Intraflagellar transport (IFT) trains, the polymers composed of two multi-subunit complexes, IFT-A and IFT-B, carry out bidirectional intracellular transport in cilia, vital for cilia biogenesis and signaling. The IFT-A complex is composed of six subunits (IFT144, IFT140, IFT122, IFT121, IFT139 and IFT43), mediating both the retrograde trafficking (toward the base) driven by the dynein-1b and the ciliary import of various membrane proteins across the ciliary gate. Here, we purified the IFT-A complex from protozoa Tetrahymena thermophila and determined the cryo-EM structures of the IFT-A complex and its subassemblies at a resolution range of 3.6 to 8.8 Å. Analysis of these structures reveal that the apo IFT-A complex is composed of two rigid structural modules, the head and base modules, and presents two distinct–elongated and folded states in solutions, the latter of which was not identified in recent IFT-A structural studies.

In particular, IFT144, IFT140, IFT122 and IFT121, share the same domain organization, from the N- to the C-termini encompassing two tandem WD40 β-propellers (WDs), an array of 12 to 20 TPRs and, except for IFT140, a zinc binding domain (ZBD). These four subunits are distributed into the two modules; the head module consists of IFT140, IFT144 and the C-terminal half of IFT122 (IFT122C, 706-1246), whereas the base module consists of IFT121, the N-terminus of IFT122 (IFT122N, 1-705) as well as IFT139 and IFT43. In contrast to the head-module elongated conformation, the base module adopts a compact configuration. IFT121, IFT122 and IFT139 together form an enclosed oval-shaped ring with the N-terminal TPRs of IFT139 (IFT139N, 1-694) extending out in a solenoid conformation. The short linkers (~5 residues) between the WD40 propellers and the TPRs in IFT121 and IFT122 constrain the locations of the propellers right atop the IFT121-IFT122 TPR junction to form half of the oval ring. This conformation is stabilized by extensive contacts between IFT121 and IFT122, which bury ~3130 Å2 solvent exposed surface area of the base module. On the other side, the ZBD of IFT121 fits into a helical groove formed by the TPRs of IFT139, constituting the other half of the base ring. Notably, the base module oval ring is sealed by the very C-terminal residue of IFT139, Lys1334, whose aliphatic sidechain sticks into hydrophobic central cavity of IFT122WD1. A salient feature of the base module is that, IFT43, the smallest subunit of the complex, adopts an elongated configuration and traverses the base as a molecular tether to stabilize the ring-shaped architecture. The N-terminus of IFT43 (IFT43N) travels along the surface of the two WDs of IFT121 with the aromatic sidechains of Trp9-Phe11 and Trp33 deeply embedded into the hydrophobic pockets in IFT121WD1 and IFT121WD2 respectively, clamping the two propellers in a fixed orientation in the base module.

> MKCSELWTEIIPKNDPNSNITNQVWSCSFNNDGSILLACVGDAILVYDSFTGNLVNKAIRGGQKEQINCIKFSKDGKRFATASNDKTVWVWSFDVNKNPKLAPEVKYSHTDKVLCLAFNPLTHQIFSGGAQDYALWTPDQQSIEKSKFKDKIITCAWSWDGLYLGFGTMGGIIGIRNRALEQLAEIQRSFPIWCMDWTPITPDYQNSVLVVGVWEQSIAHYNIQGQQLGSDKKLTYDPIDINFSTQGEFLLVSGTNNKCTLYTREGGFLIDVATKNDWVWNNKLKPVIKEAGSVAVQDQLHVALTTNDGEISMFKIQQLTVHALEGDKYAYRDNLTDIVVQSMSSNQRIRLKCKELVKNISIYKDKLAAHLTERILIYGTSSEDSQMKYKLHKRIVKKVEAHILEIVSNHLIACVKNKVQLYQLSGDLEKEWVFDSRVNCIKIIGGMPNKEGAYVGLKNGQIFKIFVDNSFPIPILNHNISIKNIDASQKRKRLAVVDKNSNLTVYDLSNKEQVFQEMNIVSCAFNNNFDDLLAFSSTDTTFIRCSNHPPLSQKISGQVVGFKANKLFVLNDNVMSTIDVSMTQTMIKYLERKEFQSAYEISLLGVTDQDFLYLGNEALIATQFAIARKCYTRIKKLDFIYLLEKAEKDFKKNTFVEGFYQGEIYALQTKFYEAENALTKSNLASQAKEMWIILKEFDKAMRITDTGASPINRGQNKEINSDASRKDLLIQRAEWEVKQGNWKKGGELYIQAEVYKKAIEVYVTNNFSEGIVEVCRNADAETQRKEIEQCAAYFKKAKLHQYTKEAYLKLQDNKALLQLNIDLEKWDEAMTLAKAHPEFMEIVKLPYANWLAKQDRYEESLKAYRKIGKHDMATKMLYNLSQNAVFEKRFSDAALFTWMIATEHLGLIRNMKAPTPEDIENLMKFYQYRDDAEIYFAYSKVQSFVDEPFLPLSGHAYMLNIFNAARFAINKLGNRQLYGVQHSYLYYSLGKVSKQLEGYKTARICYEKLASYKIPTEWSEEIELSTLLIRSKPYSDQESLLPICNRCYNQNPALTEGNRCSSCMHQFQNCFISFENLPLVEFKLDPKITHKRFIELINSDKSKTQPNKKKKKANDGWQESHQGDQQVLTFNNSPQKGGNDNESSPFLDKLNEVFEIQQTTQEYIPVTLDENIVSSLSIDEVYWVDYTKYCYTAEIKYYKSMLTDIPLKNCQECGTFYILDEYEFEISKTQKCPFCRSVDERAGPQKDVFDF;> MFVFLSKKIGMPNNAKIEAVCWNKEQGWIAAGGEKGILKVLKIEDQRQKDGSNPTTTGQLLVNNTLEYHTSNVYLVTWNDRYRKLTSVEENGIIVVWAYFRELQLWKEEMINDRKKSVVRDLKWSPDGQKVCIAYEDGAVIVGSVEGSPLWRKEFPHKLALIEWSPDSKMMIFGTPEGEVRVYDSQGMEMQRLKIHCLQKLIDPSKSFSPDLPLAAIDWFPQAKMYTDDTPPGLCIAYQCGRVQLMKNEKDDEPVLIDTMMKIFTVKWNPSGSMFAISGTQDENGELKGVVQFYSNAGHHLKTLRVPGSDRVTGVSWEGSGLRIAMAVNQAIFFANIKPDHKWAYMSDGTLAFAYQKIDRVEYTIIFWDTINNKKNLKFVKNLCCLRASGDLCCIVTELIGYDLWQIDLCNSIGSPIDSKQINIYPNAVTMTKTHIIVCSQDHVYAWQYKNQVERLTTFEQQTGLRRVGREQAWFIDKENDSNNQYDKDTYDVEPQSEDVICTVAANENFLLVARISGTINVYTFPHISLENKLHIQTRPSQMSLNKDATRLAIIDHNGNLNILKITPQGDELLPFEKKECWFVKYSDDIPESFVFMERSRMYIVNDQTPEEPIITEGYICQYKDFQVKIVYLDDIMKSPDGVLRKEELTLEIEANILKDIKDQLYKKSMQEMFIVIKQHDNDCLWRVYAKKALEDNDFDSAENAFVQCKDYASLKFLQRVRELDDRERQRAEIQCYFNKVEEAEEIYNKIERRDLSIQMRMKLGDWAQVVDQIREGTGQDVELQKARLELGNYYAENFQWDKAAKQYALAKYNPGLIEAYTRIQDYEGLEKLIAEIPERNELLQDMGDRFQQAGLCDAAVKCYEKFGDIKQAIDCCVLLNHWNLAVELAEQYNFVQIEGLLVQYANQLLEKRRKLEAAELYRKAKRNTEAAKILSQIADDLTERDANPLNIKKMYVMAALEVDLYKKRMLDATMTGQATSTAKTLNSLITSTINTSSADKILNNPWRGAEAWHFFILAQRQLYNGQFKYALKSALRLGEYELEIDQKKIYSLIAIAAYYNKSFRECSRAFVKLQNLENITEDEKERYEAIAVSIFTKHPPLDSPCEYTPCVGKNCSQQVSEYDIHCRACGSNFSPCVASGRPIFQKEFYQCKNCRHKMIESEVSRLKLYNCALCHSPIDFKRFTESNNNNNNNI;> MQNQQQKMQTILIAQSQVYYYIREGFWSTMQRFCQEQYKAFGDPFFIFWKAYGLYQEGLPNEAINELTSIQHKKEIQYATIVALITYHLSTNIVDRETVQNLKFEESTQRRLSSDKAICLAAFFYAFNKEHAKARDLIDEIHSDNFNIRIASAWCYLLEGGKFLEKSVQLFEELYNEQHEINKNLESLMGRSKANEMIKKFDISLNTINEINVLYPDFKGGLIEKAKLLMTVDDWEQLVDYCNKILYDDDKNIMALMLLTFYTFAREGDIETGCERLQKLIQAVEFSESRNMQLMFKISQVFSRISGRNTQILKFTMKLVNQCKQLSPLNAQYFCELAQQLLMVNQFERAEQYFQEASAIDVDNKECLMGLILSKIMQGQTEDAESQIDFINQTTNNGERTSEIAYLEALVSTKQENVDPRVTIKLLEESLKLHIAQANRLYPSFDFYIVLNPDFLMSLSQAYFFQVGMKEMLAGKQPQNGVASKGTKLLDFIIKKIPGLIPAYLLQAKGKMSMGNTQEALKSVTKVIEQDPKNEEAYILSAMIASSSKNFSLAQNQLQQALSNNFMIRDNPLFMLVKGEVEYAQGSYQACLETMKAAYEIPEVKDKANQSKVVSAMSVLQFSDKDRCSIFLLYAKALQQNNNSKEAKKIMTQAISQFTGTTEEVNVLIANSEIALQSGDVKKAISILKGVPQESPYFLRARQILADVYLDQLRDRRNYAKCYADLIEIDPSFDNYKMLGDALMKIREPEEASRAYEKAALIKPDDEQIIQLLGLSLCQTHDYNKALTYYENALRMNPKRLDLIIDLGKLCIQIKNFNRAEEILKPDIFSDEYQLPTYQNLKRNQEGFYLIAKLNIKRTPPGVFTPIDMYRKALKKSIQIQIDVIEKAKQEGEDVEKERKTLADMYIELAKYTNQYEKNEKATLDILAEASKYTNNQDTMSKTVGNQEKILELEVQMYFKSNQKLECENKCNLLLKLNPNNDLACLTLAELLLQKDEYSQAIEQFKKILQDRPNNYGILAKLIDFFRRSFQINEAKTYIERAEKKATNTNDPGLCYCRGLYHKYNRSPKDALNEFSKAKKSSQYAEESLVNMIDIYLNPDQDLYYSNVEEGPKVVDEVNLRACESLLREMQIRASYLRYIVMESYVFFLGGPRYKGGLEQGLKNLNDILKTNNDYIPAMLALAVGKFIQKKSTDAKNLLKLLWKRQYTTEYGEDLERAWLLSADSFIAIQKYDSAEEILKKCLKYNQSCGKAEEYMGLIKEKEQSYVDAATHYEKAYKLTNEKSASIAFRLSFNYLKAKRYVDCINICKKILVLFPNYPKIEKDCLEKARQALK;> MAAKGKQGWGFGGKDQNVKIDTSQQDQKKQNIWEQNNEDLIFVPDLTQEAQEQEVSKVSAPPNQPTVQVQDINELQKFTKINTLPQTEEGVDLSQLMQILSPVEDIKEKDEAWEFLQLKTQIYEIVSNMYGGNELIDDDDEDDENQ> MFMYSVFTCRYWRYIMVRLIKHQQLLGEYCMNVSIEEFTHFDFQLVPEPSPLDLVITESLKNHIEVNGVKSGALLPLPFQTGIGKTYTALNFLLQQMLEQVRSELKEENTGKKSKRLLYYVTDSVDNVVSAKADLLKLIEKQTVKGEPRFTLEQQEYLKAQIVHLPNQSEQLLQCSDAVLNDVLIGFNLNAERDVQAEWSAISGLRRHASNPEVKISLNRQAGYFYRNLIDRLQKKQKGADRVLLSGSLLASVETLLPGEKIRNGSAHVAFLTTSKFLKGFHNTRSRYSPLRDLSGAVLIIDEIDKQNQVILSELCKQQAQDLIWAIRTLRANFRDHQLESSPRYDKIEDLFEPLRERLEEFGTNWNLAFAFNTEGANLNERPVRLFSDRSFTHVSSATHKLSLKSDFLRRKNLIFSDEKVEGSLIEKHGLLTRFVNEADVIYQWFLGTMRKAVFQYWENVRGLEIEVRENRSLEGTFQEAVQSLLTHFNLQEFESAVYESFDTRGLRQSAGGKANKLSSSKSYHHTGLKLVEVAHNQGTRDTVNCKASFLNTSPSGVLADMVDAGAVILGISATARADTVIHNFDFKYLNERLGNKLLSLSREQKQRVNNYYHSRRNYKDNGVVLTVKYLNSRDAFLDALLEEYKPEARSSHFILNHYLGIAESEQAFVRSWLSKLLASIKAFISSPDNRYMLSLLNRTLDTTRQNINDFIQFCCDKWAKEFNVKTKTFFGVNADWMRLVGYDEISKHLNTELGKVVVFSTYASMGAGKNPDYAVNLALEGESLISVADVTYSTQLRSDIDSIYLEKPTQLLLSDDYSHTANQLCQF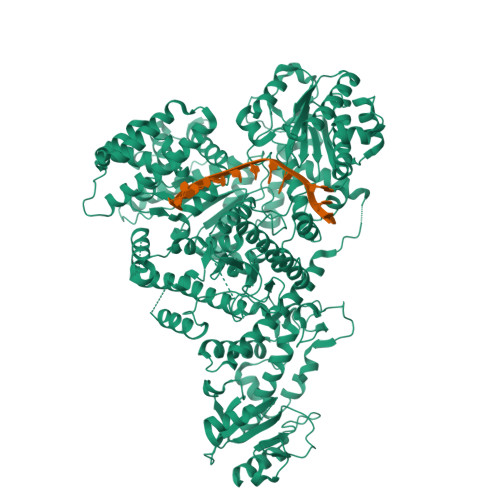HQILSLQENGELSPKSAENWCRQQLMGMSRERSLQQYHQTSDYQSAVRKYIEQAVGRAGRTSLKRKQILLFVDSGLKEILAEESRDPSLFSHEYVALVNKAKSAGKSIVEDRAVRRLFNLAQRNNKDGMLSIKALVHRLHNQPASKSDIQEWQDIRTQLLRYPTVAFQPERFNRLYLQSMTKGYYRYQGNLDGDPNSFEFFDRVPYGDMVSEEDCSLATLVQNQYVRPWFERKGFACSWQKEANVMTPIMFTNIYKGALGEQAVEAVLTAFDFTFEEVPNSIYERFDNRVIFAGIEQPIWLDSKYWKHEGNESSEGYSSKIALVEEEFGPSKFIYVNALGDTSKPIRYLNSCFVETSPQLAKVIEIPALIDDSNADTNRTAVQELIKWLHHS> QCDNFPQMLRDLRDAFSRVKTFFQTKDEVDNLLLKESLLEDFKGYLGCQALSEMIQFYLEEVMPQAENQDPEAKDHVNSLGENLKTLRLRLRRCHRFLPCENKSKAVEQIKNAFNKL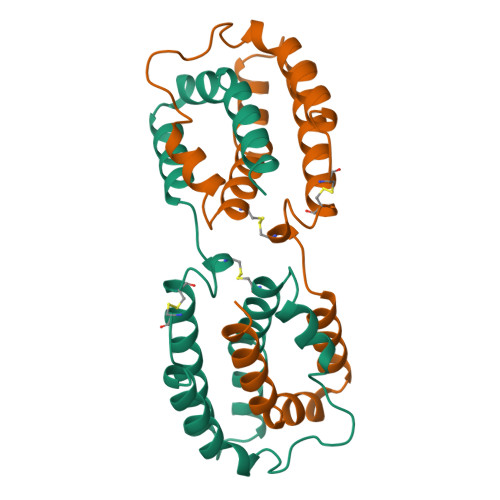QEKGIYKAMSEFDIFINYIEAYMTIKAR>MHSAANAKQQKHFVLVHGGCLGAWIWYKLKPLLESAGHKVTAVDLSAAGINPRRLDEIHTFRDYSEPLMEVMASIPPDEKVVLLGHSFGGMSLGLAMETYPEKISVAVFMSAMMPDPNHSLTYPFEKYNEKCPADMMLDSQFSTYGNPENPGMSMILGPQFMALKMFQNCSVEDLELAKMLTRPGSLFFQDLAKAKKFSTERYGSVKRAYIFCNEDKSFP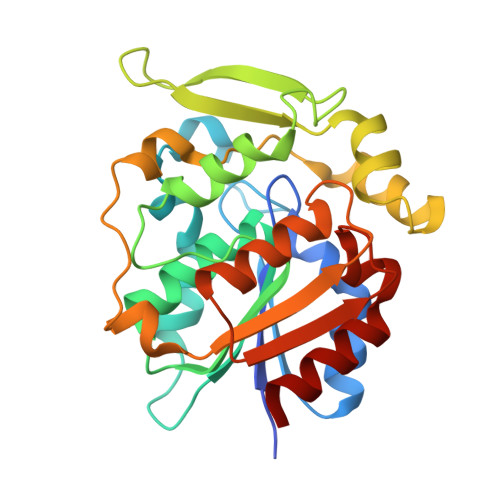VEFQKWFVESVGADKVKEIKEADAMGMLSQPREVCKCLLDISDS[5x]>MPDELKPHFANVQAHYDLSDDFFRLFLDPTQTYSCAYFERDDMTLQEAQIAKIDLALGKLGLQPGMTLLDVGCGWGATMMRAVEKYDVNVVGLTLSKNQANHVQQLVANSENLRSKRVLLAGWEQFDEPVDRIVSIGAFEHFGHERYDAFFSLAHRLLPADGVMLLHTITGLHPKEIHERGLPMSFTFARFLKFIVTEIFPGGRLPSIPMVQEC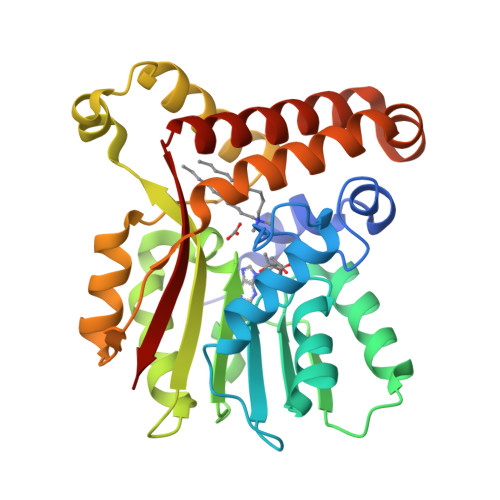ASANGFTVTRVQSLQPHYAKTLDLWSAALQANKGQAIALQSEEVYERYMKYLTGCAEMFRIGYIDVNQFTCQK[4x]> MAHHHHHHMNHDQSHALFSRAQQLLPGGVNSPVRAFKSVGGEPFFVERADGAYLYDVDGNRYIDYVGSWGPMIVGHNHPAVRQAVKKAIDNGLSFGAPCAGEVTMAETITRLVPSCEMVRMVNSGTEATLSAIRLARGATGRNRIVKFEGCYHGHGDS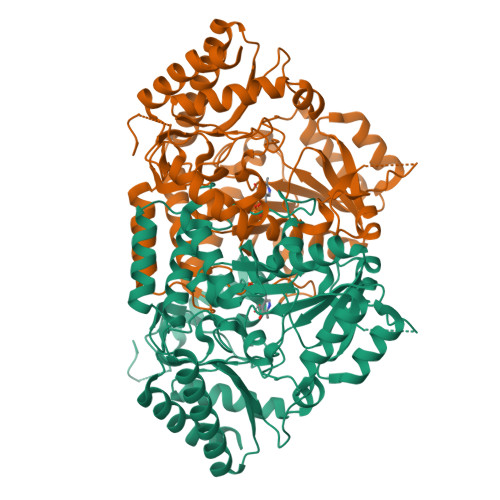FLVKAGSGMLTLGVPTSPGVPAGLSELTLTLPYNDFEAATALFEQQGDDIAGLIIEPVVGNANCIPPREGYLQHLRALCTKHGALLIFDEVMTGFRVALGGAQAHYGITPDLTTFGKIIGGGMPVGAYGGRRELMQQIAPAGPIYQAGTLSGNPVAMAAGLAMLELVQQPGFHADLAERTARLCAGLEAAAADAGVAVTTTRVGAMFGLFFTSEKVETYAQATACDIPAFNRFFHAMLEQGVFLAPSAYEAGFLSSAHDDAVIEATLAAARVAFRAAKG> GDQLTHVVEEVKTYDLVWRSIKNLWEDVQRTFETPWCRVDVLLLQSDLANFLRRADELPRAVKQFEMYKSLFSQVNMLTSVNKILVELKDGALKPRHWNMIFRDIGKRQIQKNLLDKLEFSLKDVMVLNLTLNEILLTKIIERAQKEFVIEKSLNRIKKFWKEAQYEVIEHSSGLKLVREWDVLEQACKEDLEELVSMKASNYYKIFEQDCLDLESKLTKLSEIQVNWVEVQFYWLDLYGILGENLDIQNFLPLETSKFKSLTSEYKMITTRAFQLDTTIEVIHIPNFDTTLKLTIDSLKMIKSSLSTFLERQRRQFPRFYFLGNDDLLKIIGSGKHHDQVSKFMKKMFGSIESIIFFEDSITGVRSVEGEVLNLNEKIELKDSIQAQEWLNILDTEIKLSVFTQFRDCLGQLKDGTDIEVVVSKYIFQAILLSAQVMWTELVEKCLQTNEFSKYWKEVDMKIKGLLDKLNKSSDNVKKKIEALLVEYLHFNNVIGQLKNCSTKEEARLLWAKVQKFYQKNDTLDDLNSVFISQSGYLLQYKFEYIGIPERLIYTPLLLVGFATLTDSLHQKYGGCFFGPAGTGKTETVKAFGQNLGRVVVVFNCDDSFDYQVLSRLLVGITQIGAWGCFDEFNRLDEKVLSAVSANIQQIQNGLQVGKSHITLLEEETPLSPHTAVFITLNPGYNGRSELPENLKKSFREFSMKSPQSGTIAEMILQIMGFEDSKSLASKIVHFLELLSSKCSSMNHYHFGLRTLKGVLRNCSPLVSEFGEGEKTVVESLKRVILPSLGDTDELVFKDELSKIFDSAGTPLNSKAIVQCLKDAGQRSGFSMSEEFLKKCMQFYYMQKTQQALILVGKAGCGKTATWKTVIDAMAIFDGHANVVYVIDTKVLTKESLYGSMLKATLEWRDGLFTSILRRVNDDITGTFKNSRIWVVFDSDLDPEYVEAMNSVLDDNKILTLPNGERLPIPPNFRILFETDNLDHTTPATITRCGLLWFSTDVCSISSKIDHLLNKSYEALDNKLSMFELDKLKDLISDSFDMASLTNIFTCSNDLVHILGVRTFNKLETAVQLAVHLISSYRQWFQNLDDKSLKDVITLLIKRSLLYALAGDSTGESQRAFIQTINTYFGHDSQELSDYSTIVIANDKLSFSSFCSEIPSVSLEAHEVMRPDIVIPTIDTIKHEKIFYDLLNSKRGIILCGPPGSGKTMIMNNALRNSSLYDVVGINFSKDTTTEHILSALHRHTNYVTTSKGLTLLPKSDIKNLVLFCDEINLPKLDKYGSQNVVLFLRQLMEKQGFWKTPENKWVTIERIHIVGACNPPTDPGRIPMSERFTRHAAILYLGYPSGKSLSQIYEIYYKAIFKLVPEFRSYTEPFARASVHLYNECKARYSTGLQSHYLFSPRELTRLVRGVYTAINTGPRQTLRSLIRLWAYEAWRIFADRLVGVKEKNSFEQLLYETVDKYLPNQDLGNISSTSLLFSGLLSLDFKEVNKTDLVNFIEERFKTFCDEELEVPMVIHESMVDHILRIDRALKQVQGHMMLIGASRTGKTILTRFVAWLNGLKIVQPKIHRHSNLSDFDMILKKAISDCSLKESRTCLIIDESNILETAFLERMNTLLANADIPDLFQGEEYDKLLNNLRNKTRSLGLLLDTEQELYDWFVGEIAKNLHVVFTICDPTNNKSSAMISSPALFNRCIINWMGDWDTKTMSQVANNMVDVVPMEFTDFIVPEVNKELVFTEPIQTIRDAVVNILIHFDRNFYQKMKVGVNPRSPGYFIDGLRALVKLVTAKYQDLQENQRFVNVGLEKLNESVLKVNELNKTLSKKSTELTEKEKEARSTLDKMLMEQNESERKQEATEEIKKILKVQEEDIRKRKEVVMKSIQDIEPTILEAQRGVKNIKKQQLTEIRSMVNPPSGVKIVMEAVCAILGYQFSNWRDIQQFIRKDDFIHNIVHYDTTLHMKPQIRKYMEEEFLSDPNFTYETINRASKACGPLYQWVNAQINFSKVLENVDPLRQEMKRIEFESLKTKANLLAAEEMTQDLEASIEVSKQKYSLLIRDVEAIKTEMSNVQANLDRSISLVKSLTFEKERWLNTTKQFSKTSQELIGNCIISSIYETYFGHLNERERGDMLVILKRLLGKFAVKYDVNYRFIDYLVTLDEKMKWLECGLDKNDYFLENMSIVMNSQDAVPFLLDPSSHMITVISNYYGNKTVLLSFLEEGFVKRLENAVRFGSVVIIQDGEFFDPIISRLISREFNHAGNRVTVEIGDHEVDVSGDFKLFIHSCDPSGDIPIFLRSRVRLVHFVTNKESIETRIFDITLTEENAEMQRKREDLIKLNTEYRLKLKNLEKRLLEELNNSQGNMLENDELMVTLNNLKKEAMNIEKKLSESEEFFPQFDNLVEEYSIIGKHSVKIFSMLEKFGQFHWFYGISIGQFLSCFKRVFIKKSRETRAARTRVDEILWLLYQEVYCQFSTALDKKFKMIMAMTMFCLYKFDIESEQYKEAVLTMIGVLSESSDGVPKLTVDTNDDLRYLWDYVTTKSYISALNWFKNEFFVDEWNIADVVANSENNYFTMASERDVDGTFKLIELAKASKESLKIIPLGSIENLNYAQEEISKSKIEGGWILLQNIQMSLSWVKTYLHKHVEETKAAEEHEKFKMFMTCHLTGDKLPAPLLQRTDRVVYEDIPGILDTVKDLWGSQFFTGKISGVWSVYCTFLLSWFHALITARTRLVPHGFSKKYYFNDCDFQFASVYLENVLATNSTNNIPWAQVRDHIATIVYGGKIDEEKDLEVVAKLCAHVFCGSDNLQIVPGVRIPQPLLQQSEEEERARLTAILSNTIEPADSLSSWLQLPRESILDYERLQAKEVASSTEQLLQEM;> GMTNWQQQLPLTDTQKNELDKSVLRYLNWNYKQTVRHEHAQDYESVRHAIVTLSGFLLQESVDRQEFISNNDTSNESMVDIDELLLPKKWNSIVRLQKKIIELEQNTETLVSQIKDLNTQVSELAQFKPTTSNGTSAHNVLKWIPRNLPSCLINVESSVTSVKLHPNLPIVFVATDHGKLYAFDLFNYTIPLASLQSHTKAITSMDVLFTNYTNSSKKNYLVIVTASKDLQIHVFKWVSEECKFQQIRSLLGHEHIVSAVKIWQKNNDVHIASCSRDQTVKIWDFHNGWSLKTFQPHSQWVRSIDVLGDYIISGSHDTTLRLTHWPSGNGLSVGTGHEFPIEKVKFIHFIEDSPEIRFRTPSTDRYKNWGMQYCVSASRDRTIKIWEIPLPTLMAHRAPIPNPTDSNFRCVLTLKGHLSWVRDISIRGQYLFSCADDKSVRCWDLNTGQCLHVWEKLHTGFVNCLDLDVDFDSNVTPRQMMVTGGLDCKSNVFMR

Cytoplasmic dynein-1 (dynein) is a highly conserved molecular motor that moves toward the microtubule minus end, transporting various cargoes including RNAs, membrane vesicles, and viruses, and plays a crucial role in cell division. Dynein belongs to the ATPase associated with various cellular activities (AAA+) family of proteins. Its heavy chain features a motor domain composed of six AAA+ modules, a long stalk, a microtubule-binding domain (MTBD) located at the end of the stalk, a buttress region that makes additional connections between the AAA5 module and the stalk, and a long tail that interacts with dynactin and an activating adapter. Lis1 is a dimer (~90 kDa) with an amino-terminal dimerization domain and carboxy-terminal β-propellers that bind to the dynein motor domain24,25. Our data support a model in which Lis1 relieves dynein autoinhibition by increasing its basal ATP hydrolysis rate and promoting conformations compatible with complex assembly and motility.

We also prepared grids with samples that were pre-incubated with Lis1 before ATP addition. Because some of our maps showed partial density for the Lis1 β-propellers, we performed 3D classifications without alignment in Relion to further resolve this compositional heterogeneity. This analysis distinguished states with no, one, or two Lis1 β-propellers bound to dynein. The nucleotide occupancies in these new maps correspond to the nucleotides observed in pre-3D classification maps. In addition, the interaction sites between Lis1 and dynein in our maps are those previously characterized and are largely the same in the bent and intermediate dynein states. Previous low-resolution data showed that dynein in a strong microtubule-binding state binds one Lis1 β-propeller at sitering. Our straight linker map also had one Lis1 β-propeller bound. Aligning straight linker dynein with or without Lis1 by AAA1 shows that the linker shifts slightly to accommodate Lis1 binding. In our straight linker dynein bound to one Lis1 at sitering, the density for the AAA5 loop is missing, but it is present in the intermediate or bent linker structures bound to one or two Lis1.>[8x]MSFTYKRLDKNDAAVLFVDHQAGLLSLVRDFSPDEFKNNVLALADIARFFNLPTILTTSFEDGPNGPLVPELKEMFPQAPYIARPGNINAWDNEDFVKAVKATGKKQLIIAGVVTDVCVAFPTLSALEEGFDVFVVTDASGTFNPVVRDAAWARMTAAGAQLMNWFSVGCELHRDWRNDIEGFGAILGGHLPAYANLIQSFGTKK

YcaC belongs to the isochorismatase-like protein family, which is a group of cysteine hydrolases known to work on vinyl ethers, conjugated primary amides and lactams. The crystal structure of the monomer consists of a central six-strand parallel beta-sheet with alpha-helices on both sides and three C-terminal helices that interact with the neighboring monomer. The quaternary structure is an octameric cylinder, which is built from two stacked tetramers. The pin-wheel arrangement of YcaC appears to be vital to the function of the more closely-related enzymes, since each putative active site is made up of residues from one chain and the C-terminus of the neighboring chain.

P. aeruginosa YcaC crystallized in two space groups with identical crystal morphology and similar resolution limits. In the crystal form II structure, the active site Cys118 is covalently modified to form an S-mercaptocysteine, while in the crystal form I structure, Cys118 is linked to a propanamide. Most likely, the reducing agent used in the crystallization, tris(2-carboxyethylphosphine) (TCEP), acted as a catalyst for the phosphine-catalyzed addition of excess acrylamide from the preparative native gel electrophoresis to the nucleophilic thiol of Cys118. The propanamide has a hydrogen bond to Ser59 at a distance of 3.0–3.1 Å, which supports the idea that acylamide is an accidental suicide substrate for a nucleophilic thiol. We have ascertained that the putative catalytic residue is indeed nucleophilic and reacts with electrophiles. Crystal form I also has one 2,5-hexanediol bound per sub-unit in the interface between subunits. The ligand density is poorly defined, and most of the interaction appears to be hydrophobic, but there are hydrogen bonds to residues Pro192, Asn196 or Glu71 of the neighboring chain. While the active site interaction between neighboring subunits is contained within the pin-wheel tetramer, the hexanediol binding bridges the dimerization of tetramers. Furthermore, one sulfate ion per monomer is located at a salt bridging distance from the stacked guardinium head groups of Arg7 and Arg174.> MELTDEEASFLTRRQLLALSENGDLPDDIEYEVDLDLKFANNRLKRAYIALQAWKKAFYSDPFNTAANWVGPDVCSYKGVFCAPALDDPSVLVVAGIDLNHADIAGYLPPELGLLTDVALFHVNSNRFCGVIPKSLSKLTLMYEFDVSNNRFVGPFPTVALSWPSLKFLDIRYNDFEGKLPPEIFDKDLDAIFLNNNRFESTIPETIGKSTASVVTFAHNKFSGCIPKTIGQMKNLNEIVFIGNNLSGCLPNEIGSLNNVTVFDASSNGFVGSLPSTLSGLANVEQMDFSYNKFTGFVTDNICKLPKLSNFTFSYNFFNGEAQSCVPGSSQEKQFDDTSNCLQNRPNQKSAKECLPVVS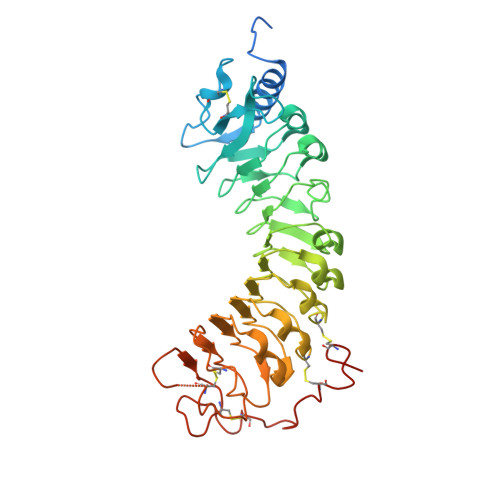RPVDCSKDKCAGGLEGSENL>[4x]AAGAPKPPQEPDMNNLPENPIPQHQAKFVLNTIKAVKRNREAVPFLHPVDTVKLNVPFYYNYIPRPMDLSTIERKINLKAY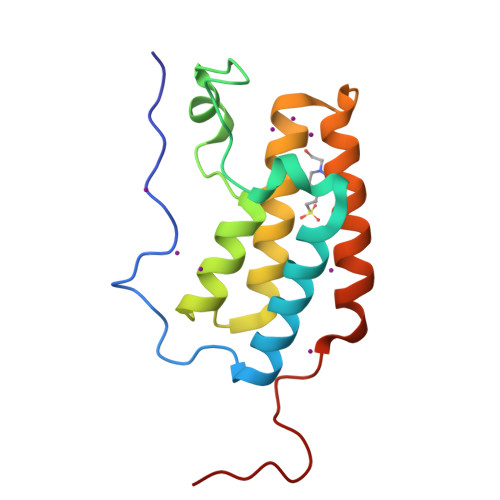EDVSQVVDDFNLMVKNCKKFNGEAAGISKMATNIQAQFEKLMVKVPPKELPAGTNVA>GAGAGAGAGAQTVKPFKEGDRAVFLGNSITDGGRYHSFIWLYYMTRFPNMPIRVFNGGIGGDTAYDMNKRLDGDIFSKNPTVLMVTFGMNDSGYYEYNGDNAKEFGEQKY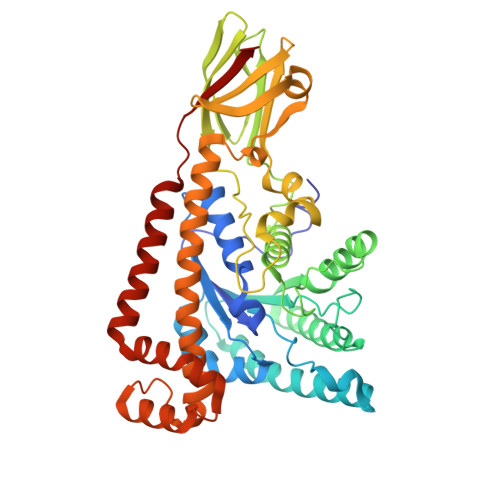QESIKNFQQMEKRFKELPHTRIVMTGTSPYDETAQIKDNTVFKKKNETIKRIIEYQRESAARNGWEFTDWNAPMVAINQELQQKDPSFTLCGNDRIHPDNDGHMVMAYLFLKAQGFAGKDVANMEINANKKQAVKAEGCTISNIKKIGKDISFDYLAEALPYPLDTIARGWGSKKSQAEVIKEVPFMEEMNTELLKVTGLKGQYKLLIDDQEIGTWDAADLAKGINLAAESKTPQYQQALTIMHLNEYRWELERTFREYAWCQFGFFQQKGLLFANDRKAIEVMDENVEKNMWLKGRRDLYSKMMFKEIRDAREQEMDVLISKIYEINKPVVRKIVLRKI[4x]> MAYVEIIEQPKQRGMRFRYKCEGRSAGSIPGERSTDTTKTHPTIKINGYTGPGTVRISLVTKDPPHRPHPHELVGKDCRDGYYEADLCPDRSIHSFQNLGIQCVKKRDLEQAISQRIQTNNNPFHVPIEEQRGDYDLNAVRLCFQVTVRDPAGRPLLLTPVLSHPIFDNRAPNTAELKICRVNRNSGSCLGGDEIFLLCDKVQKEDIEVYFTGPGWEARGSFSQADVHRQVAIVFRTPPYADPSLQAPVRVSMQLRRPSDRELSEP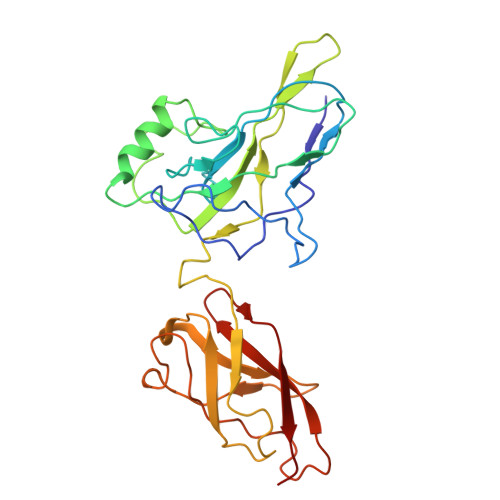MEFQYLPD>DNSYKMDYPEMGLCIIINNKNFHKSTGMTSRSGTDVDAANLRETFRNLKYEVRNKNDLTRE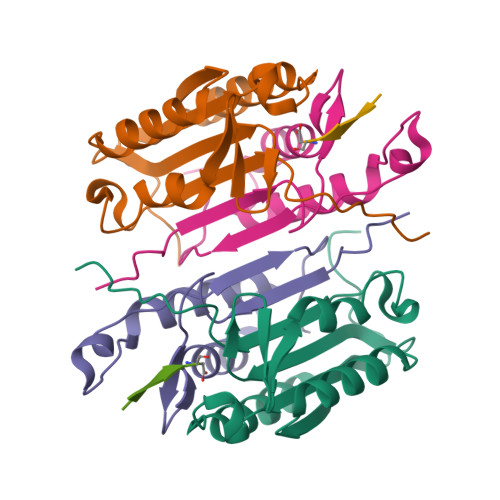EIVELMRDVSKEDHSKRSSFVCVLLSHGEEGIIFGTNGPVDLKKITNFFRGDRCRSLTGKPKLFIIQACRGTELDCGIET[2x];>CHKIPVEADFLYAYSTAPGYYSWRNSKDGSWFIQSLCAMLKQYADKLEFMHILTRVNRKVATEFESFSFDATFHAKKQIPCIVSMLTKELYFYHH[2x];>XVDFVD[2x]3,4-difluorophenyl 2-deoxy-2-[(difluoroacetyl)amino]-beta-D-glucopyranoside | C14 H15 F4 N O6 | 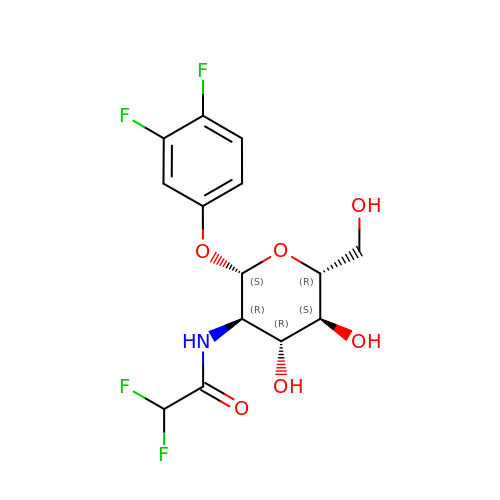YFQSDCPFGCAUBD-GOBQNSBTSA-N>MALAKRIDAALILKDGRVVKGSNFENLRDSGDPVELGKFYSEIGIDELSFWDITASVEKRKTMLELVEKVAEQIDIPITVGGGIYDFETASELILRGADKVEINTAAVENPSLITQIAQTFGSQAVVVYIAAKRVDGEFMVFTYSGTKNTGILLRDWVVEVEKRGAGEIVLGSIDRLGTKSGYDTEMIRFVRPLTTLPIIAHRGAGKTEHFLEAFLAGADAAKADSVFHSREIDVRELKEYLKKHGVNVRLEGLGS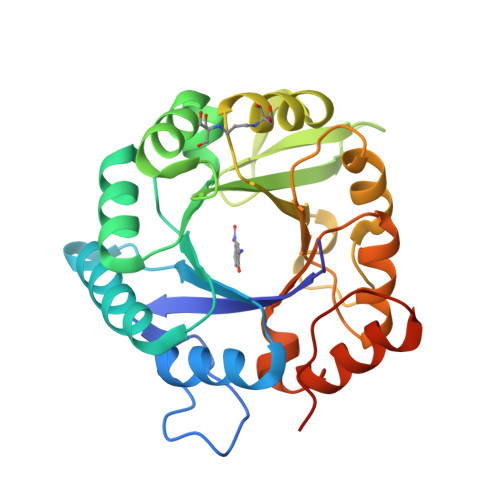LEHHHHHH[12x]> XAP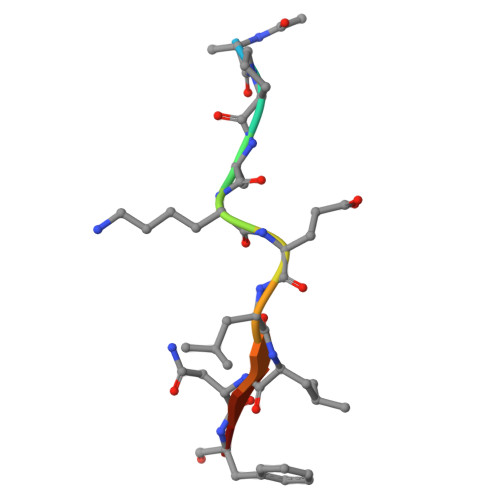AKELLNFD> SNAVTGTKVITNQVRLSFVHVLEPHAMEEGQEKKYSCMLIIPKDDKETLKAMKEAIKTAYEGAKGDKLKGVKFERLKTTLRDGDEEMDTEE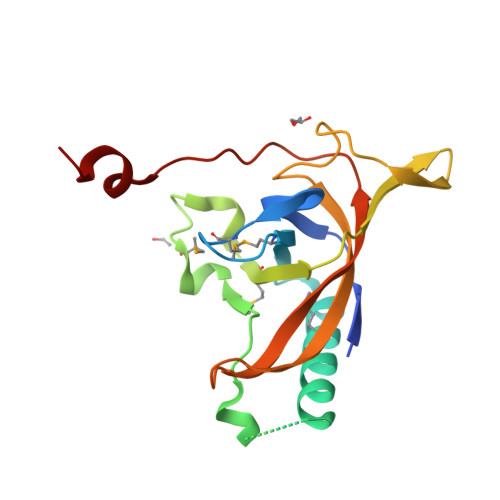RPEFENAMFINVSSKTKPQVVKREDGVLVKTDDPDEVYSGVYAIASINFYAYSTAGNKGVTAGLNNILTLCKGDFLGGRANAESDFGDL N-[3-[(4R,5R,6R)-2-azanyl-5-fluoranyl-4,6-dimethyl-5,6-dihydro-1,3-thiazin-4-yl]-4-fluoranyl-phenyl]-5-(fluoranylmethoxy)pyrazine-2-carboxamide | C18 H18 F3 N5 O2 S | 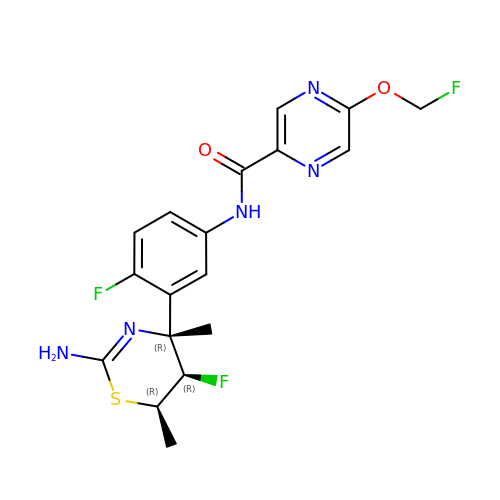JWJQXZNLFNMIHE-AHRODOEDSA-N> 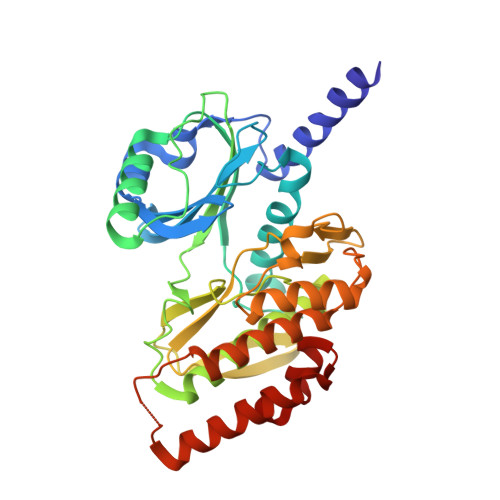LGSIEISNKKASDAEKVYGECSQKGPVPFSHCLPTEKLQRCEKIGEGVFGEVFQTIADHTPVAIKIIAIEGPDLVNGSHQKTFEEILPEIIISKELSLLSGEVCNRTEGFIGLNSVHCVQGSYPPLLLKAWDHYNSTKGSANDRPDFFKDDQLFIVLEFEFGGIDLEQMRTKLSSLATAKSILHQLTASLAVAEASLRFEHRDLHWGNVLLKKTSLKKLHYTLNGKSSTIPSCGLQVSIIDYTLSRLERDGIVVFCDVSMDEDLFTGDGDYQFDIYRLMKKENNNRWGEYHPYSNVLWLHYLTDKMLKQMTFKTKCNTPAMKQIKRKIQEFHRTMLNFSSATDLLCQHSLFK>MEYKSSPKRPYLLRAYYDWLVDNSFTPYLVVDATYLGVNVPVEYVKDGQIVLNLSASATGNLQLTNDFIQFNARFKGVSRELYIPMGAALAIYARENGDGVMFEPEEIYDELNIEPDTEQPTGFYEAVD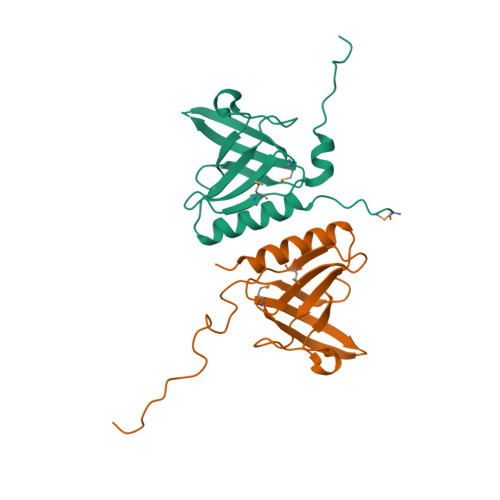[2x]> MVSLPRMVYPQPKVLTPCRKDVLVVTPWLAPIVWEGTFNIDILNEQFRLQNTTIGLTVFAIKKYVAFLKLFLETAEKHFMVGHRVHYYVFTDQPAAVPRVTLGTGRQLSVLEVRAYKRWQDVSMRRMEMISDFCERRFLSEVDYLVCVDVDMEFRDHVGVEILTPL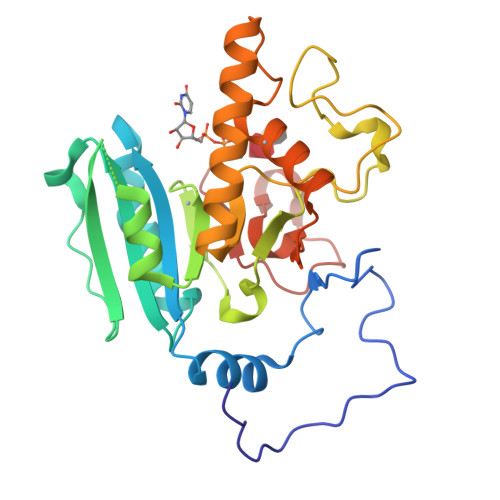FGTLHPGFYGSSREAFTYERRPQSQAYIPKDEGDFYYLGRFFGGSVQEVQRLTRACHQAMMVDQANGIEAVWHDESHLNKYLLRHKPTKVLSPEYLWDQQLLGWPAVLRKLRFTAVPKNHQAVRNP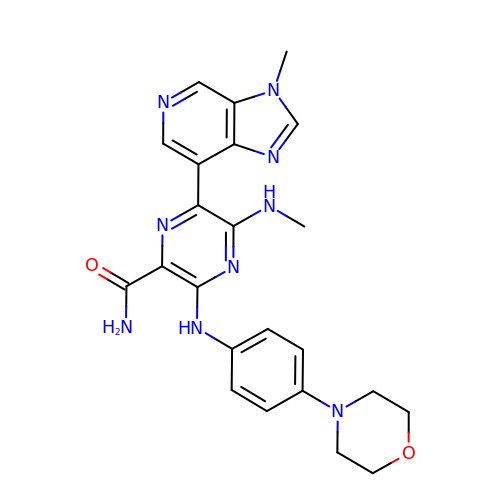5-(methylamino)-6-(3-methylimidazo[4,5-c]pyridin-7-yl)-3-[(4-morpholin-4-ylphenyl)amino]pyrazine-2-carboxamide | C23 H25 N9 O2 | LHHRWQSZVGBCHK-UHFFFAOYSA-N> GPGHMVVKFSYMWTINNFSFCREEMGEVIKSSTFSSGANDKLKWCLRVNPKGLDEESKDYLSLYLLLVSCPKSEVRAKFKFSILNAKGEETKAMEDQRAYRFVQGKDWGFKKFIR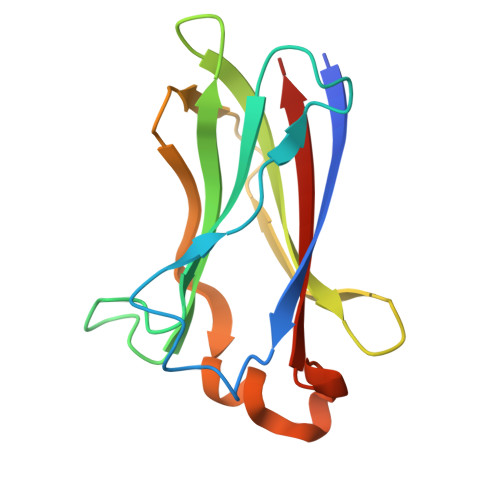RDFLLDEANGLLPDDKLTLFCEVSVVQD> MALLPDKEKLLRNFLRCANWEEKYLYIIELGQRLPELRDEDRSPQNSIQGAQSQVWIVMRQNAQGIIELQGDSDAAIVKGLIAVVFILYDQMTPQDIV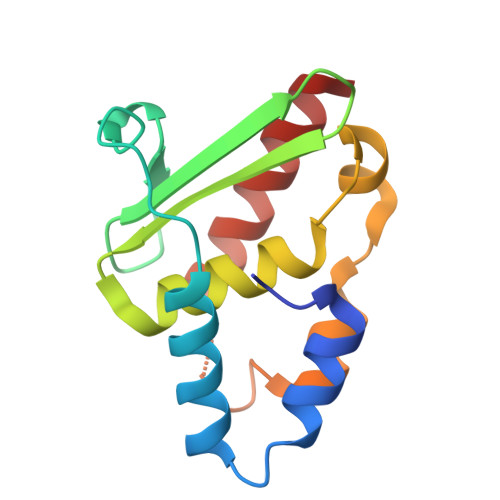NFDVRPWFCKMALTQHLTPSRSQGLEAMIRAIRAKAAALS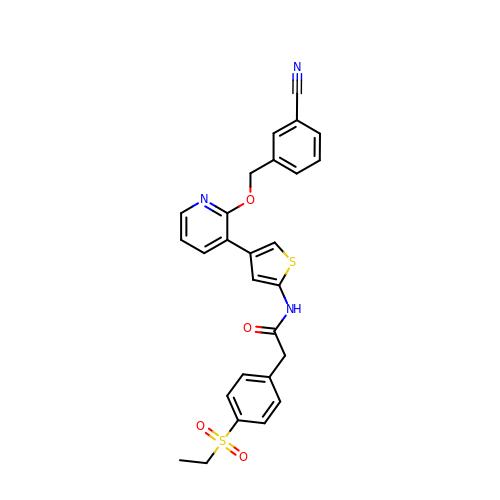~{N}-[4-[2-[(3-cyanophenyl)methoxy]pyridin-3-yl]thiophen-2-yl]-2-(4-ethylsulfonylphenyl)ethanamide | C27 H23 N3 O4 S2 | JXRNAZFJZOAFOB-UHFFFAOYSA-N> ADNYAATRYPIILVHGLTGTDKYAGVLEYWYGIQEDLQQRGATVYVANLSGFQSDDGPNGRGEQLLAYVKTVLAATGATKVNLVGHSQGGLTSRYVAAVAPDLVASVTTIGTPHRGSEFADFVQGVLAYDPTGLSSTVIAAFVNVFGILTSSSNNTNQDALAALKTLTTAQAATYNQNYPSAGLGA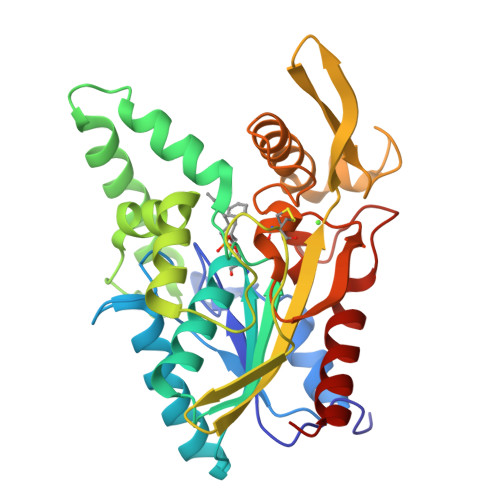PGSCQTGAPTETVGGNTHLLYSWAGTAIQPTISVGGVTGATDTSTIPLVDPANALDPSTLALFGTGTVMVNRGSGQNDGVVSKCSALYGQVLSTSYKWNHLDEINQLLGVRGANAEDPVAVIRTHANRLKLAGV> MLTVLGRLLERNSIYVATIFGGAFAFQGFFDVAVNKWWEEHNKAKLWKNVKGKFLEGEG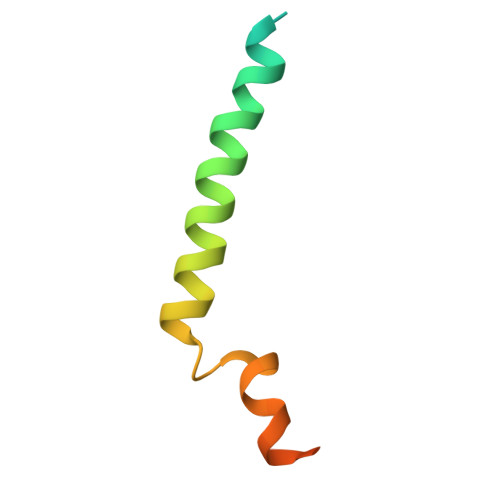EEEDDE>NQPVNQPILAAAQSLHREATKWSSKGNDIIAAAKRMALLMAEMSRLVRGGSGTKRALIQCAKDIAKASDEVTRLAKEVAKQCTDKRIRTNLLQVCERIPTISTQLKILSTVKATMLGRTNISDEESEQATEMLVHNAQN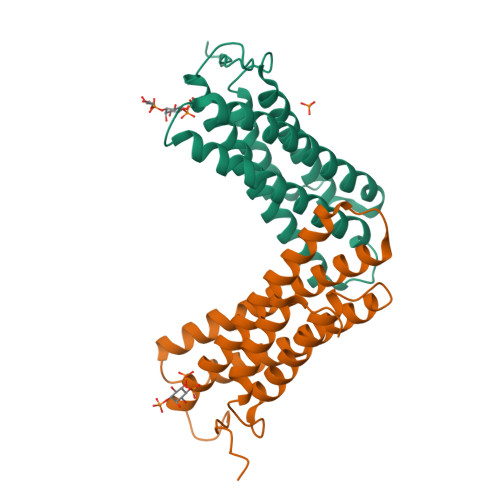LMQSVKETVREAEAASIKIRTDAGFTLRWVRKTPWYQ[4x]>GSAPADNAADARPVDVSVSIFINKIYGVNTLEQTYKVDGYIVAQWTGKPRKTPGDKPLIVENTQIERWINNGLWVPALEFINVVGSPDTGNKRLMLFPDGRVIYNARFLGSFSNDMDFRLFPFDRQQFVLELEPFSYNNQQLRFSDIQVYTENIDNEEIDEWWIRGKASTHISDIRYDHLSSVQPNQNEFSRITVR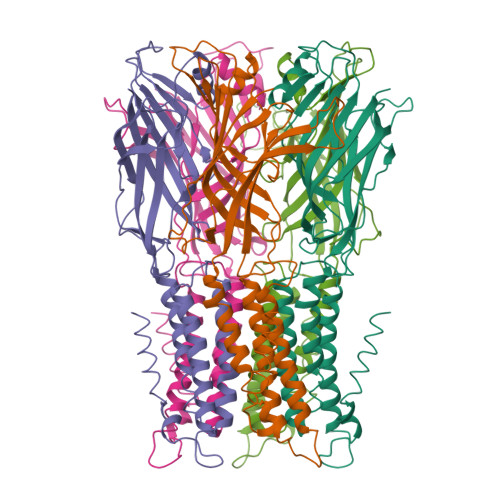IDAVRNPSYYLWSFILPLGLIIAASWSVFWLESFSERLQTSFTLMATVVAYALYTSNILPRLPYTTVIDQMIIAGYGSIFAAILLIIFAHHRQANGVEDDLLIQRCRLAFPLGFLAIGCVLVIRGITL[10x]NF-κB proteins are characterized by a Rel homology region (RHR) that supports DNA binding and assembly of homodimers and heterodimers. RelA and Rel are the most closely related NF-κB family members. One specialized function of the NF-κB Rel protein in macrophages is activation of Il12b, which encodes a key regulator of T cell development. Thus, Rel-dependent Il12b induction does not reflect a distinct motif preference but rather a heightened intrinsic DNA-binding affinity of Rel homodimers that is important for functional interactions at a subset of NF-κB sites.

To understand the difference in DNA affinity between Rel and RelA, we solved the structure of the mouse RelA(C46) chimera homodimer bound to a consensus NF-κB motif. The structures of RelA(C46) (green) and RelA (cyan) were very similar. However, the orientation of the second monomer (monomer B, right) showed significant differences in the RelA and RelA(C46) complexes in comparison with the Rel complex. Furthermore, the direct DNA-binding surface residues of RelA(C46) and RelA were nearly identical. Thus, the different affinities are unlikely to be due to differences in the DNA-binding surface. We identified Rel-specific residues on the RelA(C46) structure. None of these Rel-specific residues contacted DNA directly. Notably, the residue most likely to contribute to the increased binding affinity of mammalian Rel was Arg101, a sole residue in cluster III. The positively charged Arg101 is located behind the L1 loop, and its long side chain and guanidinium head form a network of hydrogen bonding interactions (dashed lines) with the backbone carbonyl groups on the L1 loop. This interaction could stabilize the three Arg residues of the L1 loop (Arg16, Arg18 and Arg 24) in a favorable conformation for DNA binding.

>MPYVEIIEQPKQRGMRFRYKCEGRSAGSIPGERSTDTTKTHPTIKINGYTGPGTVRISLVTKDPPHRPHPHELVGKDCRDGYYEAEFGPERRPLFFQNLGIRCVKKKEVKEAIILRISAGINPFNVPEQQLLDIEDCDLNVVRLCFQVFLPDEHGNFTTALPPIVSNPIYDNRAPNTAELKICRVNRNSGSCLGGDEIFLLCDKVQKEDIEVYFTGPGWEARGSFSQADVHRQVAIVFRTPPYADPSLQAPVRVSMQLRRPSDRELSEPMEFQYLPD[8x]> D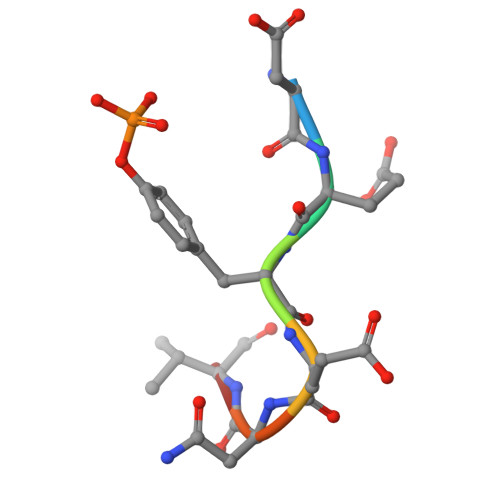EYENVD>[2x]QCVKLNDGHFMPVLGFGTYAPPEVPRSKALEVTKLAIEAGFRHIDSAHLYNNEEQVGLAIRSKIADGSVKREDIFYTSKLWSTFHRPELVRPALENSLKKAQLDYVDLYLIHSPMSLKPGEELSPTDENGKVIFDIVDLCTTWEAMEKCKDAGLAKSIGVSNFNRRQLEMILNKPGLKYKPVCNQVECHPYFNRSKLLDFCKSKDIVLVAYSALGSQRDKRWVDPN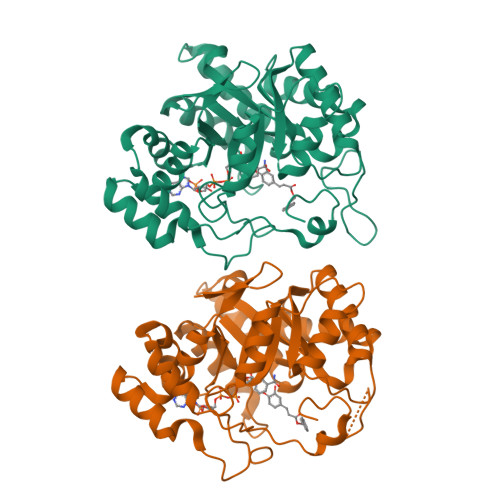SPVLLEDPVLCALAKKHKRTPALIALRYQLQRGVVVLAKSYNEQRIRQNVQVFEFQLTAEDMKAIDGLDRNLHYFNSDSFASHPNYPYS> MKLAVAGKGGVGKTTVAAGLIKIMASDYDKIYAVDGDPDSCLGQTLGL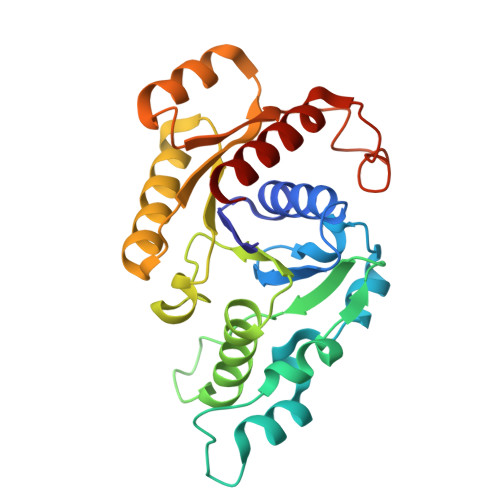SIEEAYAITPLIEMKDEIREKTGDGGLLILNPKVDGDLDKYGRYIDDKIFLIRMGEIKKGGSQCYCRENSFLGSVVSALFLDKKEAVVMDMGAGIEHLTRGTAKAVDMMIAVIEPNLNSIKTGLNIEKLAGDLGIKKVRYVINKVRNIKEEKLIKKHLPEDKILGIIPYNELFIELSLKGEEIWQSTNPAFVNLHDIYQKLRLEVG>[8x]KGGWFGKHRGQGGSNPKFENIAEGLRALLARSHVERTTDEGTWVAGVFVYGGSKTSLYNLRRGTALAIPQCRLTPLSRLPFGMAPGPGPQPGPLRESIVCY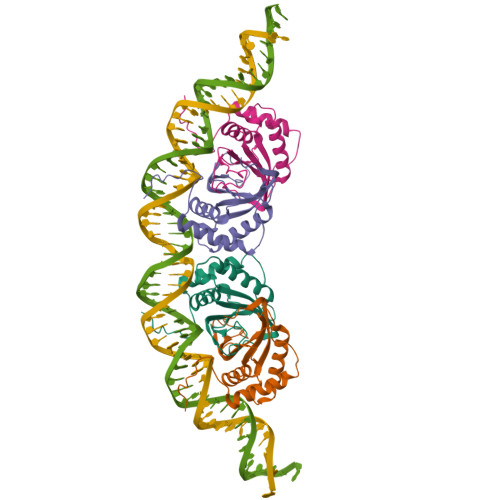FMVFLQTHIFAEVLKDAIKDLVMTKPAPTCNIRVTVCSFDDGVDLP>TEAQKCNLQGQWRNKLGSNLIIESVSQNGEFTGTYFTSVSLTNSTIRISPLTGYQKLTEKPTFGFTVHWAFSDSITVWTGQCFLNEKGEEILHTMWLLRSSQEK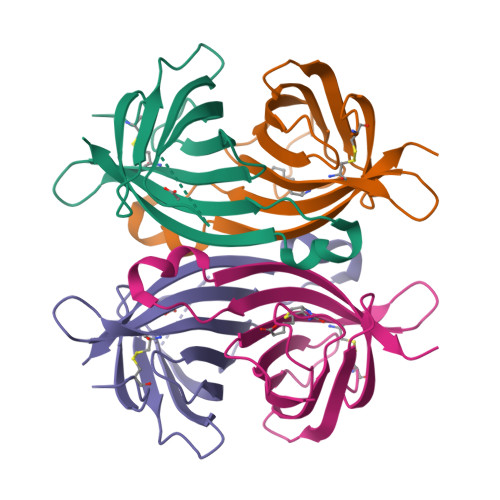EQDNWTGTRVGANTFTRLSKKKIRKE[2x]>GASTGDSFETRFEKMDNLLRDPKSEVNSDCLLDGLDALVYDLDFPALRKNKNIDNFLSRYKDTINKIRDLRMKAEDYEVVKVIGRGAFGEVQLVRHKSTRKVYAMKLLSKFEMIKRSDSAFFWEERDIMAFANSPWVVQLFYAFQDDRYLYMVMEYMPGGDLVNLMSNYDVPEKWARFYTAEVVLALDAIHSMGFIHRDVKPDNMLLDKSGHLKLADFGTCMKMNKEGMVRCDTAVGTPDYISPEVLKSQGGDGYYGRECDWWSVGVFLYEMLVGDTPFYADSLVGTYSKIMNHKNSLTFPDDNDISKEAKNLICAFLTDREVRLG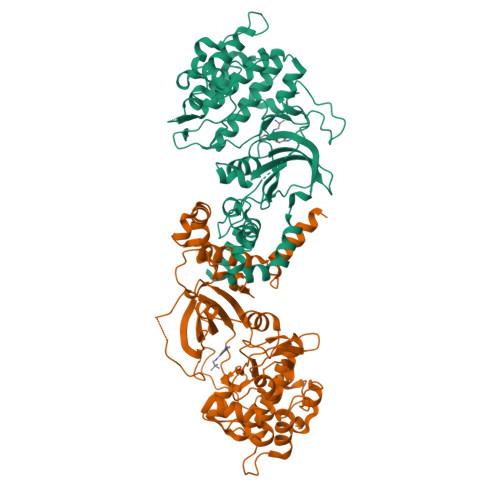RNGVEEIKRHLFFKNDQWAWETLRDTVAPVVPDLSSDIDTSNFDDLEEDKGEEETFPIPKAFVGNQLPFVGFTYYSNRRYLSSAN[4x]Human transglutaminase 2 (TG2), a member of a large family of enzymes that catalyze protein crosslinking, plays an important role in the extracellular matrix biology of many tissues and is implicated in the gluten-induced pathogenesis of celiac sprue. The catalytic mechanism, related to that of cysteine proteases, involves an active site thiol that reacts with a glutamine side chain of a protein or peptide substrate to form a thioester intermediate from which the acyl group is transferred to an amine substrate. In the absence of a suitable amine, water can act as an alternative nucleophile, leading to deamidation of the glutamine residue to glutamate. Its catalytic activity requires millimolar Ca2+ concentrations and is inhibited by guanine nucleotides. Human TG2 consists of four domains: an N-terminal β-sandwich (which, in contrast to previously solved TG2 structures, is fully resolved here) that binds to fibronectin; the catalytic domain containing a Cys-His-Asp catalytic triad; and two C-terminal β-barrels belonging to the fibronectin Type III CATH superfamily.

We have trapped human TG2 in complex with an inhibitor that mimics inflammatory gluten peptide substrates and have solved, at 2-Å resolution, its x-ray crystal structure. Ac-P(DON)LPF-NH2 is an exceptionally high-affinity irreversible inhibitor of human TG2 with inhibition parameters Ki = 60 nM and ki = 0.5 min−1. However, in contrast to an earlier structure, which showed human TG2 in a “closed” GDP-bound conformation, the inhibitor-bound structure is in an extended or “open” conformation. When the N-terminal and catalytic domains of the two structures are superimposed, the C-terminal residues are displaced by as much as 120 Å. For instance, a β-strand in the closed structure consisting of residues Leu-312 to Arg-317 becomes α-helical in the open structure, inducing backbone rearrangements that extend to the active site. The catalytic Cys (C277) is located in a hydrophobic tunnel bridged by W241 and W332, which reside on separate loops in the active site. The inhibitor, which mimics the acyl-donor substrate, occupies one side of the active-site tunnel. Notably, the inhibitor ketone is hydrogen bonded to the indole of Trp-241, as well as to the backbone amide of the catalytic cysteine, analogous to the hydrogen bonding arrangement expected for oxyanion stabilization of acylation and deacylation transition states. The penultimate (Pro) residue of the inhibitor assumes a trans configuration and orients the terminal Phe to bind in a deep hydrophobic pocket consisting of residues A304, L312, I313, F316, I331, and L420. Surprisingly, our structure reveals the existence of a vicinal disulfide bond between two surface cysteine residues, C370 and C371, which causes the intervening peptide bond to assume a cis configuration, distorting the peptide backbone.

> MAEELVLERCDLELETNGRDHHTADLCREKLVVRRGQPFWLTLHFEGRNYQASVDSLTFSVVTGPAPSQEAGTKARFPLRDAVEEGDWTATVVDQQDCTLSLQLTTPANAPIGLYRLSLEASTGYQGSSFVLGHFILLFNAWCPADAVYLDSEEERQEYVLTQQGFIYQGSAKFIKNIPWNFGQFQDGILDICLILLDVNPKFLKNAGRDCSRRSSPVYVGRVGSGMVNCNDDQGVLLGRWDNNYGDGVSPMSWIGSVDILRRWKNHGCQRVKYGQCWVFAAVACTVLRCLGIPTRVVTNYNSAHDQNSNLLIEYFRNEFGEIQGDKSEMIWNFHCWVESWMTRPDLQPGYEGWQALDPTPQEKSEGTYCCGPVPVRAIKEGDLSTKYDAPFVFAEVNADVVDWIQQDDGSVHKSINRSLIVGLKISTKSVGRDEREDITHTYKYPEGSSEEREAFTRANHLNKLAEKEETGMAMRIRVGQSMNMGSDFDVFAHITNNTAEEYVCRLLLCARTVSYNGILGPECGTKYLLNLTLEPFSEKSVPLCILYEKYRDCLTESNLIKVRALLVEPVINSYLLAERDLYLENPEIKIRILGEPKQKRKLVAEVSLQNPLPVALEGCTFTVEGAGLTEEQKTVEIPDPVEAGEEVKVRMDLVPLHMGLHKLVVNFESDKLKAVKGFRNVIIGPA> GQMAYDRAITVFSPDGRLFQVEYAREAVKKGSTALGMKFANGVLLISDKKVRSRLIEQNSIEKIQLIDDYVAAVTSGLVADARVLVDFARISAQQEKVTYGSLVNIENLVKRVADQMQQYTQYGG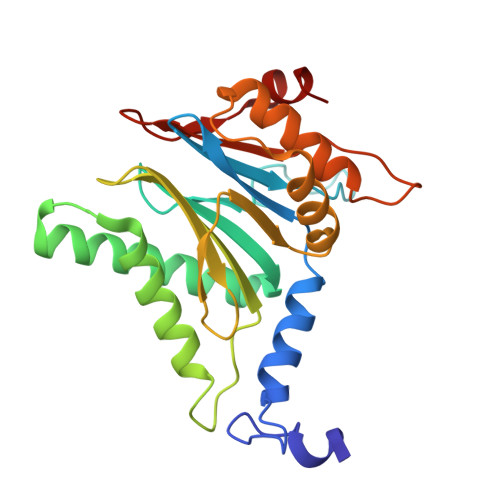VRPYGVSLIFAGIDQIGPRLFDCDPAGTINEYKATAIGSGKDAVVSFLEREYKENLPEKEAVTLGIKALKSSLEEGEELKAPEIASITVGNKYRIYDQEEVKKFL> MAGIKIIKENVDRETFEALAEICPFDAFSYENDKLEVTAACKMCKMCLKKGPEGVLILEEDEKVAIDKSLYRGITVYVDHIEGQIHPVTFELIGKARELAAVIGHPVYALLMGTNITEKADELLKYGVDKVFVYDKPELKHFVIEPYANVLEDFIEKVKPSSILVGATNVGRSLAPRVAARYRTGLTADCTILEMKENTDLVQIRPAFGGNIMAQIVTENTRPQFCTVRYKVFTAPERVNEPWGDVEMMDIEKAKLVSAIEVMEVIKKEKGIDLSEAETIVAVGRGVKCEKDLDMI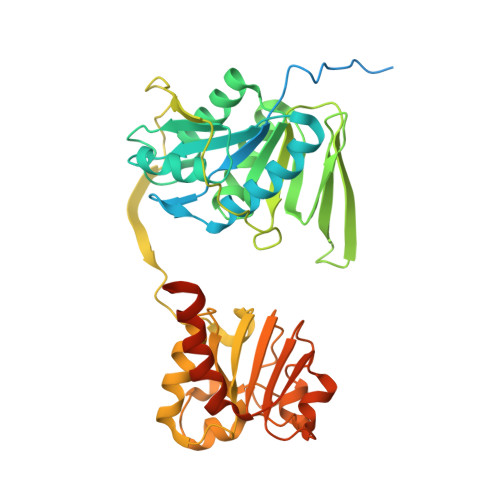HEFAEKIGATVACTRPGIEAGWFDARLQIGLSGRTVKPKLIIALGISGAVQFAAGMQNSEYIIAINSDPKAPIFNIAHCGMVGDLYEILPELLTMIEGPENNKDTETISIPEAIETPERMVV> MGGSGSRLSKELLAEYQDLTFLTKQEILLAHRRFCELLPQEQRSVESSLRAQVPFEQILSLPELKANPFKERICRVFSTSPAKDSLSFEDFLDLLSVFSDTATPDIKSHYAFRIFDFDDDGTLNREDLSRLVNCLTGEGEDTRL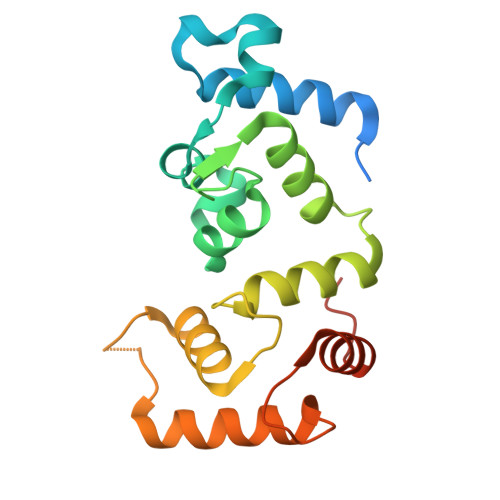SASEMKQLIDNILEESDIDRDGTINLSEFQHVISRSPDFASSFKIVL In the eukaryotic cytoplasm, Get3 delivers tail-anchored (TA) integral membrane proteins, defined by a single transmembrane helix at their C terminus, to the endoplasmic reticulum. Get3d is conserved across land plants and photosynthetic bacteria and includes a distinctive C-terminal α-crystallin domain. Distinct features of Get3d include an incomplete active site, a “closed” conformation in the apo-state, and a hydrophobic chamber. Both homologs have ATPase activity and are capable of binding TA proteins, supporting a potential role in TA protein targeting.

We solve the atomic structure of a plant Get3d and further refine a previously deposited structure of a cyanobacterial Get3d. In AtGet3d, the α-helical CBD is enclosed by additional helices not seen in the deposited Get3d structure from Nostoc sp.. With this map, we could clearly identify additional density consistent with the helices of AtGet3d that enclosed the CBD. We built into this density adding 41 residues total and further refined the NosGet3d structure with refinement statistics in Table S1. Overall, NosGet3d is structurally very similar to the AtGet3d structure (backbone RMSD = 2.33 Å). As with AtGet3d, NosGet3d has some unidentified densities in the hydrophobic chamber. One prominent difference is that the helices enclosing the CBD in NosGet3d are further from the bottom of the chamber than in AtGet3d, resulting in a larger hydrophobic chamber. In cytoplasmic Get3 proteins, it has been shown that the highly conserved aspartate in switch I coordinates a water, helping to align the water for nucleophilic attack on the γ-phosphate. This aspartate is conserved in the Get3d family, with NosGet3d uniquely having a glutamate at this position, further supporting its evolutionary drift. The catalytic aspartate in Get3, D57 in yeast, coordinates water and primes it for nucleophilic attack of the γ-phosphate of ATP. This residue is highly conserved in Get3d proteins; however, it is a glutamate in NosGet3d, which may contribute to its lower Vmax. To investigate this, the ATPase activities of AtGet3d and NosGet3d were determined by monitoring the phosphate produced by Get3d in a spectrophotometric assay. Both AtGet3d and NosGet3d were found to have ATPase activity, with a Vmax of 12.0 ± 0.1 and 3.2 ± 0.1 nmol Pi/min/mg Get3 and kcat of 1.10 ± 0.01 and 0.28 ± 0.01 min−1, respectively.

>[2x]MALILTFLGKSGVARTKIAIAAAKLLASQGKRVLLAGLAEPVLPLLLEQTLTPDPQQIAPNLEVVQFQSSVLLERNWEEVKKLEAQYLRTPIIKEVYGQELVVLPGMDSALALNAIREYDASGKYDTIVYDGTGDAFTLRMLGLPESLSWYVRRFRQLFVNSDLGKTIAESPLIQPLISSFFNVNWTADNFAQPTNQVNNFLDKGKEALADPKRVAAFLVTTADPLEVVSVRYLWGSAQQIGLTIGGVIQVSSQTEGDLSAEFTPLSVTVVPDVTKGDWQPLIDALPNFVEQAEQAPKPITIDTHNRQVRLFLPGFDKKQVKLTQYGPEVTVEAGDQRRNIFLPPALSGRPITGAKFQNNYLIISFLEHHHHHH3-deoxy-beta-D-glucopyranose | C6 H12 O5 | 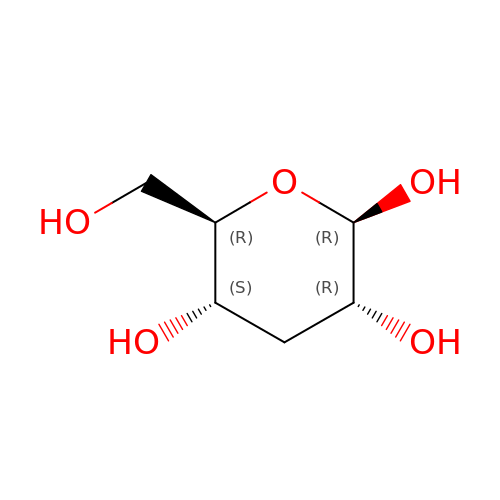RJDIFQMDPPUATQ-SLPGGIOYSA-N> MSLIARIKRFLGLEAEAKREEPEKEKSEPVGASKEEVEKVAEENAKPRIGYIHLSGCTGDAMSLTENYDILAELLTNMVDIVYGQTLVDLWEMPEMDLALVEGSVCLQDEHSLHELKELREKAKLVCAFGSCAATGCFTRYSRGGQQAQPSHESFVPIADL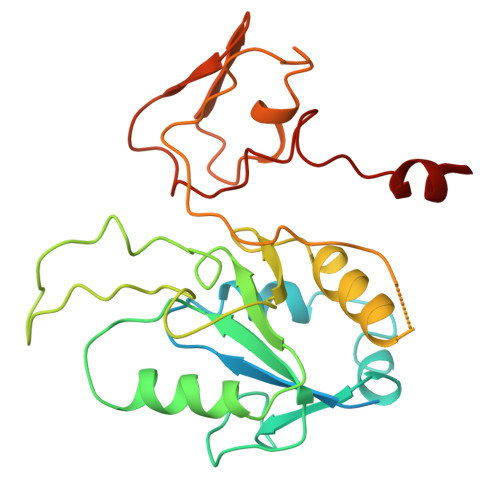IDVDLALPGCPPSPEIIAKTVVALLNNDMDYLQPMLDLAGYTEACGCDLQTKVVNQGLCIGCGTCAMACQTRALDMTNGRPELNSDRCIKCGICYVQCPRSWWPEEQIKKELGL> MKGSRIELGDVTPHNIKQLKRL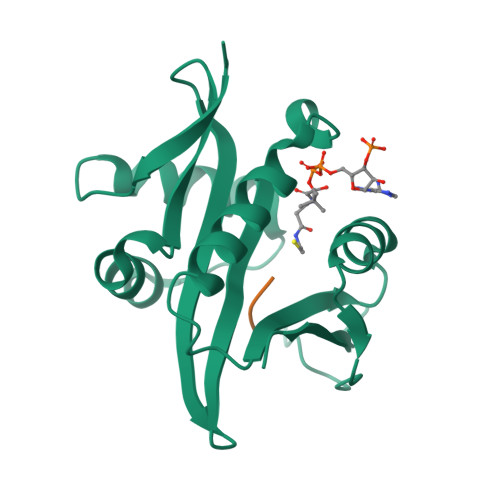NQVIFPVSYNDKFYKDVLEVGELAKLAYFNDIAVGAVCCRVDHSQNQKRLYIMTLGCLAPYRRLGIGTKMLNHVLNICEKDGTFDNIYLHVQISNESAIDFYRKFGFEIIETKKNYYKRIEPADAHVLQKNLKVPSGQNADVQKTDN;> XMMAS> TELKKVVALYDYMPMNANDLQLRKGEEYFILEESNLPWWRARDKNGQEGYIPSNYITEAEDSIEMYEWYSKHMTRSQAEQLLKQEGKEGGFIVRDSSKAGKYTVSVFAKSTGEPQGVIRHYVVCSTPQSQYYLAEKHLFSTIPELINYHQHNSAGLISRLKYPVSKQNKNAPSTAGLGYGSWEIDPKDLTFLKELGTGQFGVVKYGKWRGQYDVAIKMIREGSMSEDEFIEEAKVMMNLSHEKLVQLYGVCTKQRPIFIITEYMANGCLLNYLREMRHRFQTQQLLEMCKDVCEAMEYLESKQFLHRDLAARNCLVNDQGVVKVSDFGLSRYVLDDEYTSSVGSKFPVRWSPPEVLMYSKFSSKSDIWAFGVLMWEIYSLGKMPYERFTNSETAEHIAQGLRLYRPHLASERVYTIMYSCWHEKADERPSFKILLSNILDVMDEES

Btk is critical for the generation of calcium flux in response to receptor activation, because it activates phospholipase C-γ2 (PLC-γ2), which produces the second messengers diaceylglycerol (DAG) and inositol (1,4,5)-trisphosphate (IP3). Btk dysfunction is the cause of X-linked agammaglobulinemia, a severe disease of primary immunodeficiency. The Tec family kinases have a lipid-interaction module attached to the N terminus of a Src-like module (i.e., concatenation of an SH3 domain, an SH2 domain and a tyrosine kinase domain). The lipid-interaction module of the Tec kinases is an extended plekstrin homology (PH) domain fused to a Tec homology (TH) domain.

We determined the structure of a construct of mouse Btk spanning residues 214 to 659, which starts just before the SH3 domain and ends at the C terminus of full-length Btk. The structure resembles those described previously for autoinhibited, Src-like, non-receptor tyrosine kinases, with the SH2-kinase linker sandwiched between the SH3 domain and the small domain of the kinase (the N lobe of the kinase). The crystal structure has two molecules of Btk in the asymmetric unit, intertwined as a domain-swapped dimer in which each SH2 domain has pieces from two molecules. The domain-swapped SH2 domain packs against the large domain of the kinase (the C lobe of the kinase), but Btk lacks a Src-like C-terminal tail to stabilize this interaction. When compared with the other autoinhibited SH3-SH2-kinase structures (c-Src, Hck, c-Abl), the conserved features of the SH3/linker interaction in Btk are the polyproline type-II helix conformation adopted by residues 383–387 in the SH2-kinase linker, including the proline at position 385, and the overall hydrophobic character of the peptide-binding pocket on the SH3 domain. Diffuse electron density for the SH2 domain at every stage of our structure determination shows that this part of the polypeptide chain occupies a range of positions and adopts multiple local conformations. The unphosphorylated activation loop of Btk folds into the mouth of the catalytic cleft, blocking part of the substrate-binding site, and helix αC lies at the margin of the N lobe, preventing formation of a Glu-Lys salt bridge conserved in all catalytically active protein kinases. Glu 445, which would buttress Lys 430 in the active conformation, interacts instead with Arg 544 and Tyr 545. Leu 390 of the linker (corresponding to Trp 260 in c-Src) is sandwiched between residues Trp 421 and Tyr 461 in the kinase domain. The structure just described demonstrates that the SH3-SH2 domain in a Tec-family member can assemble into a regulatory clamp, just as it does in other Src-like kinases.>[2x]ANPCCSNPCQNRGECMSTGFDQYKCDCTRTGFYGENCTTPEFLTRIKLLLKPTPNTVHYILTHFKGVWNIVNNIPFLRSLIMKYVLTSRSYLIDSPPTYNVHYGYKSWEAFSNLSYYTRALPPVADDCPTPMGVKGNKELPDSKEVLEKVLLRREFIPDPQGSNMMFAFFAQHFTHQFFKTDHKRGPGFTRGLGHGVDLNHIYGETLDRQHKLRLFKDGKLKYQVIGGEVYPPTVKDTQVEMIYPPHIPENLQFAVGQEVFGLVPGLMMYATIWLREHNRVCDILKQEHPEWGDEQLFQTSRLILIGETIKIVIEDYVQHLSGYHFKLKFDPELLFNQQFQYQNRIASEFNTLYHWHPLLPDTFNIEDQEYSFKQFLYNNSILLEHGLTQFVESFTRQIAGRVAGGRNVP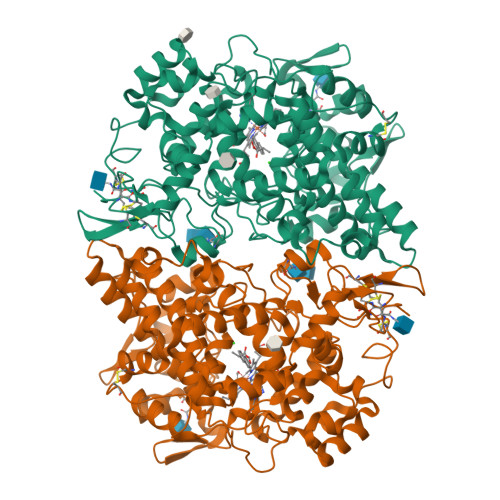IAVQAVAKASIDQSREMKYQSLNEYRKRFSLKPYTSFEELTGEKEMAAELKALYSDIDVMELYPALLVEKPRPDAIFGETMVELGAPFSLKGLMGNPICSPQYWKPSTFGGEVGFKIINTASIQSLICNNVKGCPFTSFNVQDPQPTKTATINASASHSRLDDINPTVLIKRRSTEL>MHHHHHHMSTTVEKIKAIEDEMARTQKNKATSFHLGQLKAKLAKLRRELLTSASSGSGGGAGIGFDVARTGVASVGFVGFPSVGKSTLLSKLTGTESEAAEYEFTTLVTVPGVIRYKGAKIQMLDLPGIIDGAKDGRGRGKQVIAVARTCNLLFIILDVNKPLHHKQIIEKELEGVGIRLNKTPPDILIKKKEKGGISITNTVPLTHLGNDEIRAVMSEYRINSAEIAFRCDATVDDLIDVLEASSRRYMPAIYVLNKIDSLSIEELELLYRIPNAVPISSGQDWNLDELLQVMWDRLNLVRIYTKPKGQIPDFTDPVVLRSDRCSVKDFCNQIHKSLVDDFRNALVYGSSVKHQPQYVGLSHILEDEDVVTILKK[2x];>[2x]MEQKRLERESLEKQPKITLEEFIETERGKLDKSKLTPITIANFAQWKKDHVIAKINAEKKLSSKRKPTGREIILKMSAENKSFETDNADMPDDVTQGSAWDLTEFTDALKKADHQDDGGIKDYGDGSNPTFDIKKANSATLA

The Developmentally Regulated GTP-binding proteins (DRGs) belong to the OBG family of GTPases (which also contains the Obg/CgtA, YyaF/YchF, Nog1 and Ygr210 sub-branches). In addition to the GTPase domain, these proteins also contain a C-terminal TGS domain of unknown function. The yeast Drg1 homolog is named Ribosome-binding GTPase 1 (Rbg1) as it was found associated to ribosome. It associates with yeast Dfrp1, namely Tma46, which is also a ribosome-associated protein.

The final model of the Rbg1fl–Tma46205–345 complex (R-factor 19.7%, Rfree 22.2%) includes two molecules of the complex in the asymmetric unit although the complex behaves as a heterodimer by size-exclusion chromatography. The Rbg1 structure shows a domain organization that includes the well-conserved G-domain (G1 + G2 + G3 = 64–169; G4 + G5 = 245–293), an N-terminal helix–turn–helix (HTH) domain (1–44) which lies adjacent to another domain formed by a 65-residue long insertion (176–240) between G3 and G4 of the G-domain and the TGS domain at the C-terminus (294–369). We named this new domain of Rbg1 the S5D2L domain as database searches indicate that its topology is related to the ‘Ribosomal protein S5 domain 2-like’ (S5D2L) superfamily despite the absence of significant sequence similarity. The two amphipathic helices, α1 and α2 (2–44), comprises a previously unnoticed HTH domain at the N-terminal of Rbg1. Tma46 fragment present in the structure shows a non-globular type of fold predominantly formed by α helices interconnected by coils. Tma46 helices envelops Rbg1 forming an extended and extensive interface (buried surface area in the interface ∼2978 Å2) contacting the G-domain (helices α1, α2 and ß strand) and the TGS domain (helices α3 and α4) with no contacts with the S5D2L and HTH domains. Our complex structure demonstrates that the region of Tma46 contacting Rbg1 is larger than these earlier estimates and encompasses residues 216–279 and 302–338. Interestingly, the interface between Tma46 α2 and Rbg1 α8/α9 consists mainly of aromatic ring containing residues, which form a π-stacking interaction. Superimposing human OLA1 structure bound to ATP onto the G-domain of the two chains indicated that the P-loop in chain A adopted a closed conformation where entry of GTP could be difficult whereas chain B had an open conformation.>MKGPNLTEISKKITDSNAVLLAVKEVEALLSSIDEIAAKAIGKKIHQNNGLDTENNHNGSLLAGAYAISTLIKQKLDGLKNEGLKEKIDAAKKCSETFTNKLKEKHTDLGKEGVTDADAKEAILKTNGTKTKGAEELGKLFESVEVLSKAAKEMLANSVKELTSPVVA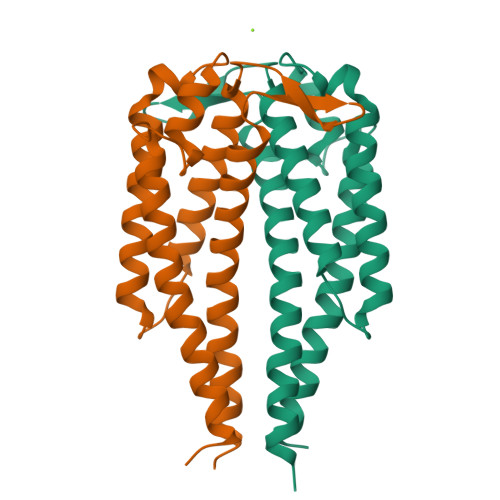ESPKKP[4x]6-[(3S)-3-(acryloylamino)pyrrolidin-1-yl]-2-{[4-(tert-butylcarbamoyl)phenyl]amino}pyridine-3-carboxamide 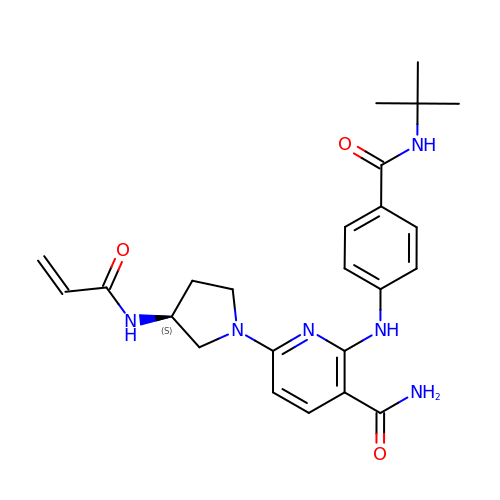| C24 H30 N6 O3 | AYRMUHGKVWLINC-KRWDZBQOSA-N> MAHAGRTGYDNREIVMKYIHYKLSQRGYEWDAGDVGAAPPGAAPAPGIFSSQPGHTPHPAASRDPVARTSPLQTPAAPGAAAGPALSPVPPVVHLTLRQAGDDFSRRYRRD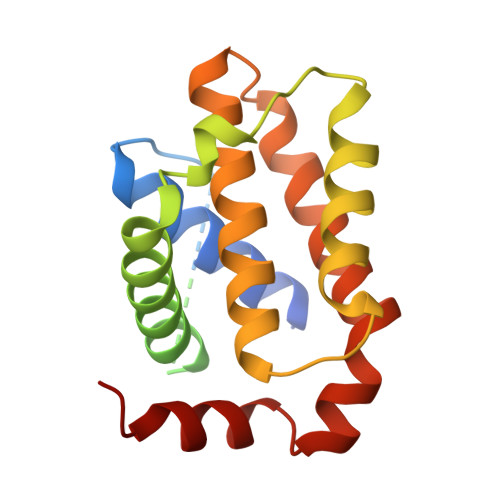FAEMSSQLHLTPFTARGRFATVVEELFRDGVNWGRIVAFFEFGGVMCVESVNREMSPLVDNIALWMTEYLNRHLHTWIQDNGGWDAFVELYGPSMR>VTLSLPNMEGRREQLIAQVESILASAADGRVQKTKETQSVDFKEEAGRRNGPQIEPGKPENPEAADKLADEVACMANTPGGGALIVGIEDKTGRIIGTELDIDWLRQGIFTRIDVAPDVVAKRVLGQRVLAIYVAAAAEPIEDTSDRLRWRVGDSCRPVDRAEWWEYQRAQSGFDPMAQVTTATLGDARPAALALARKWDPAFAELTDEELLRGIGALDAEGFLSQAGKLLFTSLDRTAIELSIFDVHGGQVLNRVVPEPEKSCLEQLDYLEQALNVVNKNNTVVEGFVHKPVPEIPRLAVREAMLNAMIHRDWNRSEPIDVRWIELDSTLIVRSPGGFPAAITSENVLSNRAARYPALADLYRALGLVDKQGVGVDRMYQAMIALGHRPPTIEEIAGPFVETTLVGGRPVLPVLELVSSIVPEARQDDYRIAIVLYLLFQRPFITIDVVARGLQSGKEAARNALEAARQTTVAGAPLIIAHDGVWLLGNACREILRKVEPSPFS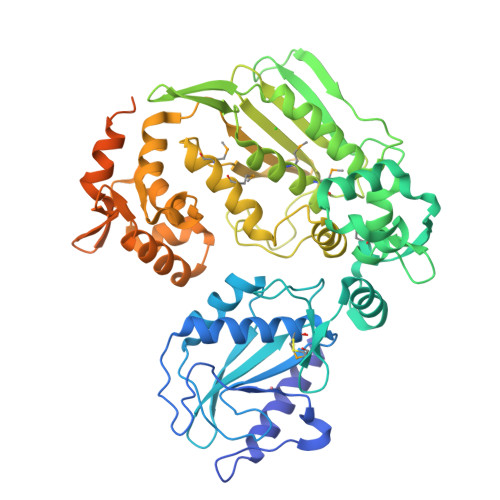PVRYLSTDQAELTNAAMLWLSEVGDLATSDLMAMCGVSRGTAKACVDGLVDEERVVAVGGGRSRRYRLVELEHHHHHH[4x]> GSHMWDAQFENLLRRYLPFLSADQPLEQDINLR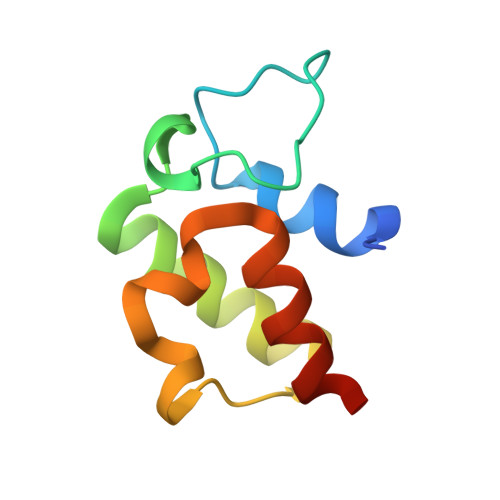DIGLDSLGTVELLSELENTYDVHFQDEALTKETFETPGVLWKTLSQMVEPRH>MDCMRKLDRVDMQLVKILSENSRLTYRELADILNTTRQRIARRIDKLKKLGIIRKFTIIPDIDKLGYMYAIVLIKSKVPSDADKVISEISDIEYVKSVEKGVGRYNIIVRLLLPKDIKDAENLISEFLQRIKNAENVEVILISEVRKFEII[2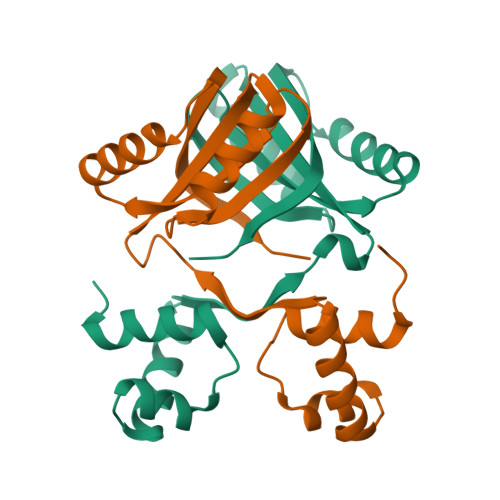x]> GSSGSSGMIKEYRTIKEVVGPLMAVEKVSGVKYEELIEVRMQNGEIRRGQVLEVQEDKAMVQIFEGTSGINYKNSSVRFLGHPLQLGVSEDMIGRVFDGLGRPKDNGPEILPEKYLDINGEVINPIARDYPDEFIQTGISAIDHLNTLVRGQKLPVFSGSGLPHKELAAQIARQATVLDSSDDFAVVFAAIGITFEEAEFFMEDFRQTGAIDRSVMFMNLANDPAIERIATPRMALTAAEYLAYEKGMHVLVIMTDMTNYAEALREISAARREVPGRRGYPGYLYTNLATLFERAGRIRGLKGSVTQIPILTMPEDDKTHPIPDLT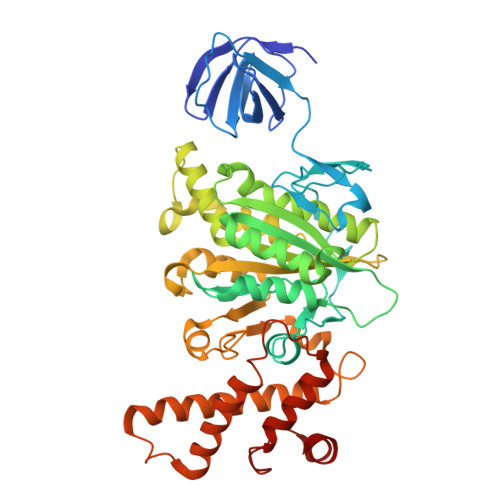GYITEGQIILTRELYKSGIQPPIDVLPSLSRLKDKGTGAGKTREDHAATMNQLFAAYAQGKQAKELAVVLGESALSDIDKIYAKFAERFENEYVNQGFYTNRTITETLDLGWELLAMLPRTELKRIKDDLLDKYLP> MGVSFKDVAGMHEAKLEVREFVDYLKSPERFLQLGAKVPKGALLLGPPGCGKTLLAKAVATEAQVPFLAMAGAEFVEVIGGLGAARVRSLFKEARARAPCIV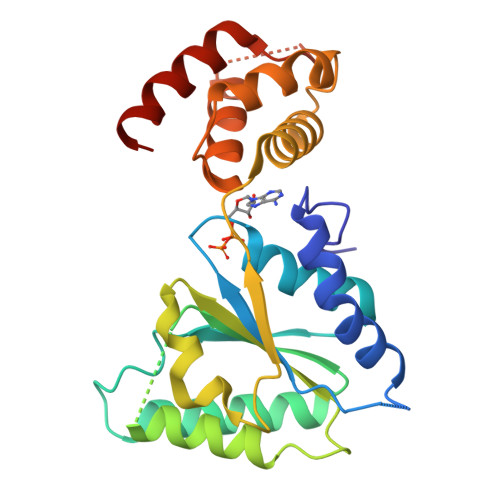YIDEIDAVGKKRSTTMSGFSNTEEEQTLNQLLVEMDGMGTTDHVIVLASTNRADILDGALMRPGRLDRHVFIDLPTLQERREIFEQHLKSLKLTQSSTFYSQRLAELTPGFSGADIANICNEAALHAAREGHTSVHTLNFEYAVERVLAGTAKKSKILSK>ADKELKFLVVDDFSTMRRIVRNLLKELGFNNVEEAEDGVDALNKLQAGGYGFVISDWNMPNMDGL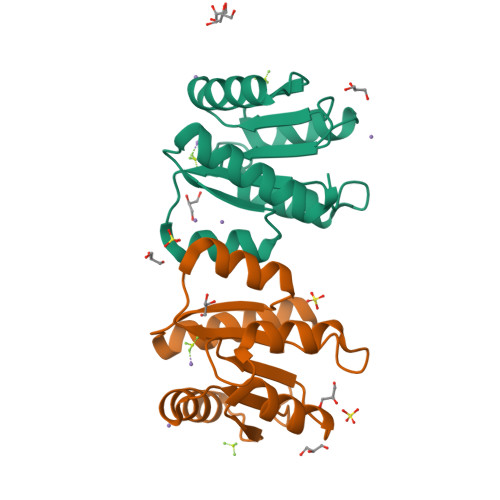ELLKTIRADGAMSALPVLMVTAEAKKENIIAAAQAGASGYVVKPFTPATLEEKLNKIFEKLGM[2x]> MEDNLINVLSINERCFLLKQSGNEKYDIKNLQAWKERKSVLKQDDLDYLIKYKYESLDNFGLGITPIENFPDKEVAIQYIKDQSWYIFFESILDSYNDSEEQLLEVDASYPFRYFLQYARLFLLDLNSELNICTKEFIINLLEILTQELIHLTSKTLVLDLHTFKKNEPLKGNDSSKRFIYYLKKRFNSKKDIIAFYTCYPELMRITVVRMRYFLDNTKQMLIRVTEDLPSIQNCFNIQSSELNSISESQGDSHSRGKTVSTLTFSDGKKIVYKPKINSENKLRDFFEFLNKELEADIYIVKKVTRNTYFYEEYIDNIEINNIEEVKKYYERYGKLIGIAFLFNVTDLHYENIIAHGEYPVIIDNETFFQQNIPIEFGNSATVDAKYKYLDSIMVTGLVPYLAMKDKSDSKDEGVNLSALNFKEQSVPFKILKIKNTFTDEMRFEYQTHIMDTAKNTPIMNNEKISFISYEKYIVTGMKSILMKAKDSKKKILAYINNNLQNLIVRNVIRPTQRYADMLEFSYHPNCFSNAIEREKVLHNMWAYPYKNKKVVHYEFSDLIDGDIPIFYNNISKTSLIASDGCLVEDFYQESALNRCLNKINDLCDEDISIQTVWLEIALNIYNPYKYINDLKNQNSNKYIYTGLELNGKIIQACQKIEKKIFKRAIFNKKTNTVNWIDIKLDQDWNVGILNNNMYDGLPGIFIFYVALKYITKNHKYDYVIECIKNSIYTIPSEDILSAFFGKGSLIYPLLVDYRLNNDINSLNVAVEIADMLIEKKPINNGELKNDWIHGHNSIIKVLLLLSEITEDEKYRKFSLEIFEKLSEEPYFNFRGFGHGIYSYVHLLSKFNRIDKANSLLHKIKESYFEEEPKNNSWCKGTVGELLATIELYDDNISNIDINKTIEYKNKDCLCHGNAGTLEGLIQLAKKDPETYQYKKNKLISYMLKYFEKNNTLKVAGSEYLESLGFFVGISGVGYELLRNLDSEIPNALLFEL

Cytolysin is produced by many clinical isolates of Enterococcus faecalis and consists of two post-translationally modified peptides termed cytolysin L and S. Cytolysin is a member of the lanthipeptides, a family of polycyclic peptides that are made in a two-step process involving dehydration of Ser and Thr residues to dehydroamino acids and subsequent addition of thiols of Cys residues to the dehydroamino acids. This process, catalyzed by the enzyme CylM for cytolysin, generates the characteristic thioether crosslinks called lanthionine (Lan) and methyllanthionine (MeLan). We describe here the 2.2 Å resolution structure of CylM and demonstrate that its dehydration domain surprisingly has structural similarity with eukaryotic lipid kinases despite the absence of notable sequence homology.

To investigate the mechanism of catalysis, we determined the 2.2 Å resolution structure of CylM in complex with adenosine monophosphate (AMP). The structure of the ∼110 kDa polypeptide consists of two distinct domains, with an N-terminal dehydration domain, composed of residues Asn4 through Pro624, and a C-terminal cyclization domain encompassed by Tyr641 through Glu992. As in NisC, CylM contains a single zinc ion near the center of the toroid coordinated by residues Cys875, Cys911, and His912, with a water molecule completing the tetrahedral coordination geometry at the metal. Although the N-terminal dehydration domain lacks detectable sequence similarities with other proteins, the CylM structure reveals that this domain is architecturally related to the catalytic core of lipid kinases, such as phosphoinositide 3-kinase (PI3K). Unlike most kinases, the activation loop in the CylM dehydration domain, composed of residues Asn365 through Val383, is well defined in the absence of bound peptide substrate. The orientation and stabilization of the activation loop is established through numerous interactions with the LanM-specific KA domain, which is itself held in place through interactions with the ‘capping helices’. In the CylM co–crystal structure, the bound AMP is located between the two lobes of the kinase domain. The phosphate-binding loop (P-loop) is composed of residues Ser247 through Thr262 and is considerably longer than the equivalent feature in PI3Ks. The adenine is situated in a hydrophobic binding pocket common across other structurally characterized kinases that is defined by CylM residues Val272 (Ile831 in PI3Kγ), Val301 (Tyr867 in PI3Kγ), Ile354 (Met953 in PI3Kγ), and Val361 (Phe961 in PI3Kγ). Inspection of the CylM structure shows that these four residues (Asp252, His254, Arg506, and Thr512) are in close proximity to each other despite a separation of >250 amino acids in primary sequence, and that they are situated in or immediately adjacent to the phosphorylation site.>MTPYAFTDPRKSELYVVEGDSAGGSAKSGRDSMFQAILPLRGKIINVEKARIDRVLKNTEVQAIITALGTGIHDEFDIGKLRYHKIVLMADADVDGQHISTLLLTLLFRFMRPLIENGHVFLAQPPLYKLKWQRSDPEFAYSDRERDGLLEAGLKAGKKINKEDGIQRYKGLGEMDAKELWETTMDPSVRVLRQVTLDDAAAADELFSILMGEDVDARRSFITRNAKDVRFLDVKLAAALEHHHHHH[2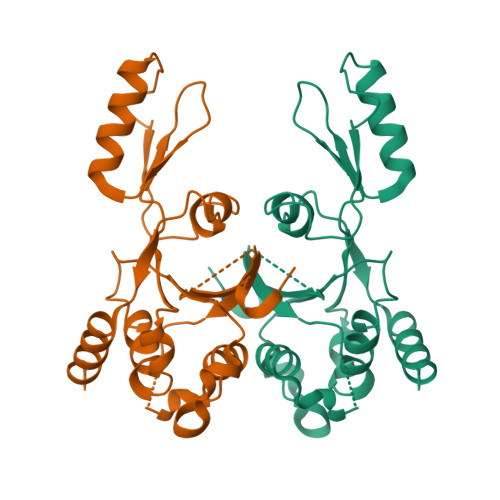x]> WDGKIDGTGTHAMIVTQGVSILENDLSKNEPESVRKNLEILKENMHELQLGSTYPDYDKNAYDLYQDHFWDPDIDNNFSKDNSWYLAYSIPDTGESQIRKFSALARYEWQRGNYKQATFYLGEAMHYFGDIDTPYHPANVTAVDSAGHVKFETFAEERKEQYKINTAGCKTNEAFYTDILKNKDFNAWSKEYARGFAKTGKSIYYSHASMSHSWDDWDYAAKVTLANSQKGTAGYIYRFLHDVSEGNDPSVGKNVKELVAYISTSGEKDAGTDDYMYFGIKTKDGKTQEWEMDNPGNDFMTGSKDTYTFKLKDENLKIDDIQNMWIRKRK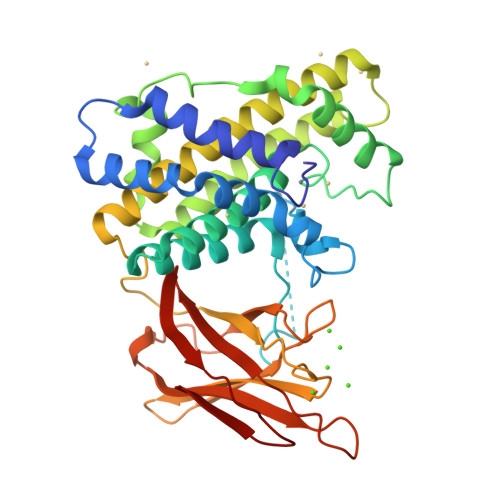YTAFPDAYKPENIKIIANGKVVVDKDINEWISGNSTYNIK>[4x]MKHLHRFFSSDASGGII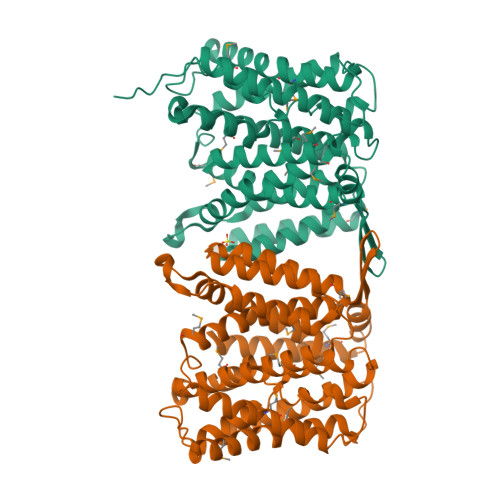LIIAAILAMIMANSGATSGWYHDFLETPVQLRVGSLEINKNMLLWINDALMAVFFLLVGLEVKRELMQGSLASLRQAAFPVIAAIGGMIVPTLLYLAFNYADPITREGWAIPAATDIAFALGVLALLGSRVPLALKIFLMALAIIDDLGAIIIIALFYTNDLSMASLGVAAVAIAVLAVLNLCGARRTGVYILVGVVLWTAVLKSGVHATLAGVIVGFFIPLKEKHGRSPAKRLEHVLHPWVAYLILPLFAFANAGVSLGGVTLDGLTSILPLGIIAGMLIGKPLGISLFCWLALRLKLAHLPEGTTYQQIMVVGILCGIGFTMSIFIASLAFGSVDPELINWAKLGILVGSISSAVIGYSWLRVRLRPSVEFRVPGSENLYFQ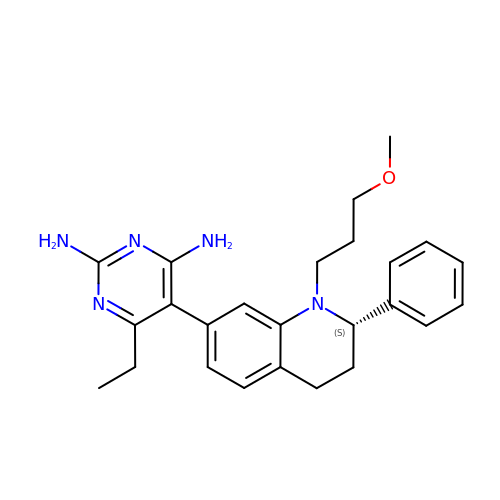6-ETHYL-5-[(2S)-1-(3-METHOXYPROPYL)-2-PHENYL-1,2,3,4-TETRAHYDROQUINOLIN-7-YL]PYRIMIDINE-2,4-DIAMINE | C25 H31 N5 O | UOYVKYJWAXJTTE-NRFANRHFSA-N(2-HYDROXYPHENYL)ACETIC 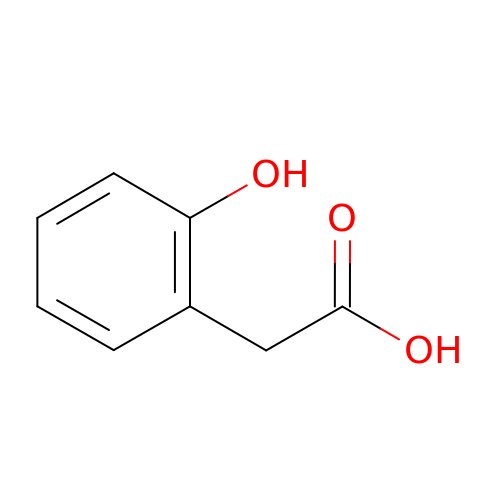ACID | C8 H8 O3 | CCVYRRGZDBSHFU-UHFFFAOYSA-N> GSICQFKLVLLGESAVGKSSLVLRFVKGQFHEYQESTIQAAFLTQTVCLDDTTVKFEIWD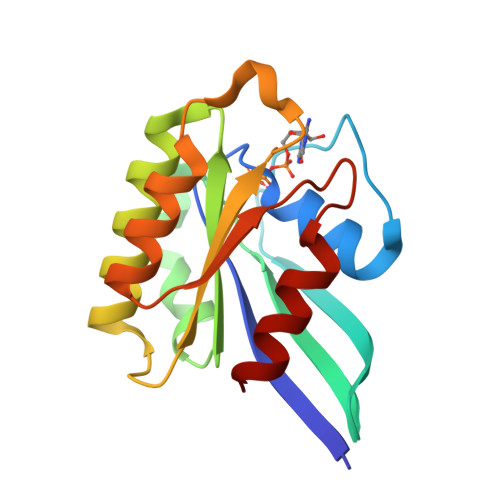TAGQERYHSLAPMYYRGAQAAIVVYDITNTDTFARAKNWVKELQRQASPNIVIALAGNKADLASKRAVEFQEAQAYADDNSLLFMETSAKTAMNVNEIFMAIAKKL>[6x]GLFDI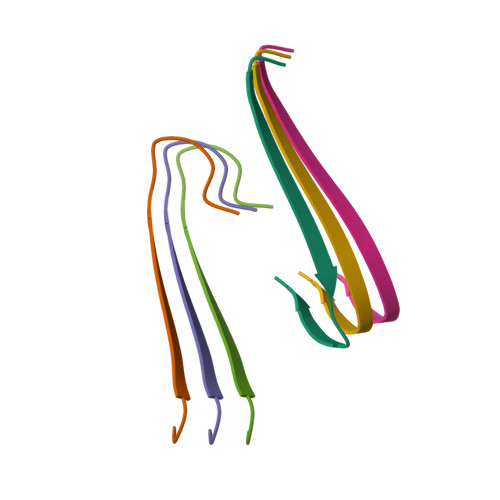IKKVASVIGGL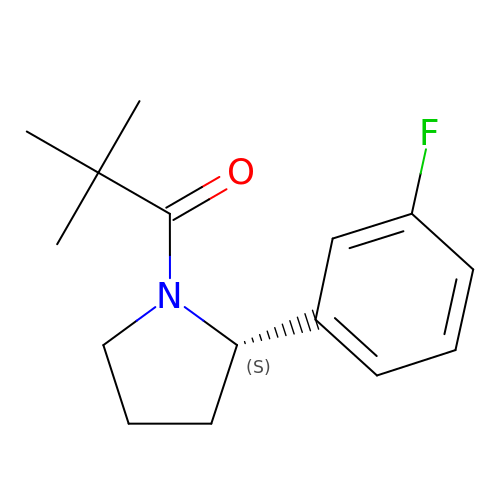1-[(2S)-2-(3-fluorophenyl)pyrrolidin-1-yl]-2,2-dimethylpropan-1-one | C15 H20 F N O | KAKAXRVKJWUSTC-ZDUSSCGKSA-N McrBC is an antiphage defense system of Escherichia coli that specifically cleaves invading DNA that are methylated. Furthermore, upon binding of the endonuclease McrC, a higher oligomeric form—tetradecamers of 12 McrB and 2 McrC protomers—is formed. GTP hydrolysis by McrBC bound to a recognition sequence powers DNA translocation, and convergence of two such complexes on the DNA results in nucleolytic cleavage. Here we present the structure of the AAA+ domain of McrB in complex with McrC at 3.6 Å resolution using cryo-electron microscopy (cryo-EM), which reveals the coupling between the endonuclease and the motor and the mechanism of activation of the GTPase.

The complex was formed in the presence of the GTP analog 5’-guanylyl imidodiphosphate (GNP). McrBΔNC is dumbbell shaped with the two hexameric McrBΔN rings tilted with respect to each other and sandwiching an McrC dimer. Three-dimensional (3D) classification resulted in nine major classes with varying tilt angle, indicative of conformational plasticity. The two protomers of McrC in the McrBΔNC complex are related to each other by a two-fold symmetry. The dimeric interface mainly constitutes helix H9 and has a total buried surface area of ~3000 Å2. The catalytic residues, Asp244, Asp257, and Lys259, are located close to the dimeric interface and aligned along the FA interface of McrB. A particularly interesting feature of McrBΔNC is that the McrC stalk blocks the pore of the McrB ring.

>MSKTESYCLEDALNDLFIPETTIETILKRLTIKKNIILQGPPGVGKTFVARRLAYLLTGEKAPQRVNMVQFHQSYSYEDFIQGYRPNGVGFRRKDGIFYNFCQQAKEQPEKKYIFIIDEINRANLSKVFGEVMMLMEHDKRGENWSVPLTYSENDEERFYVPENVYIIGLMNTADRSLAVVDYALRRRFSFIDIEPGFDTPQFRNFLLNKKAEPSFVESLCQKMNELNQEISKEATILGKGFRIGHSYFCCGLEDGTSPDTQWLNEIVMTDIAPLLEEYFFDDPYKQQKWTNKLLGDSSGSHHHHHH[12x];>[2x]MEQPVIPVRNIYYMLTYAWGYLQEIKQANLEAIPGNNLLDILGYVLNKGVLQLSRRGLELDYNPNTEIIPGIKGRIEFAKTIRGFHLNHGKTVSTFDMLNEDTLANRIIKSTLAILIKHEKLNSTIRDEARSLYRKLPGISTLHLTPQHFSYLNGGKNTRYYKFVISVCKFIVNNSIPGQNKGHYRFYDFERNEKEMSLLYQKFLYEFCRRELTSANTTRSYLKWDASSISDQSLNLLPRMETDITIRSSEKILIVDAKYYKSIFSRRMGTEKFHSQNLYQLMNYLWSLKPENGENIGGLLIYPHVDTAVKHRYKINGFDIGLCTVNLGQEWPCIHQELLDIFDEYLK Attachment of the LPyV major capsid protein VP1 to receptors on host cells is clearly critical for the restricted tropism of the virus. LPyV VP1 forms a ring-shaped homopentamer in which the five monomers are arranged around a central five-fold axis and connected by extensive interaction surfaces. Sialic acid is a crucial component of the LPyV receptor as removal or modification of cellular sialic acids abolished or modulated LPyV cell binding and infection, but the identity of the sialylated LPyV receptor and its role in tropism are not known. Glycan array and structural analyses show that LPyV VP1 specifically recognizes linear trisaccharides terminating in α2,3-linked sialic acid.

In order to elucidate the carbohydrate-binding specificity of LPyV in a controlled setting, we recombinantly expressed VP1 pentamers that are unable to assemble into capsids due to truncations of 27 and 66 residues at the N- and C-termini, respectively. The LPyV VP1 structure contains one bound Ca2+ ion per chain that is coordinated by the carboxylate group of E46 and the carbonyl group of S214cw as well as several water molecules. In addition, the carboxylate group of E217cw is close enough to the Ca2+ to engage in an ionic interaction. These residues are highly conserved among all polyomaviruses and form one of the two calcium binding sites in the SV40 virion that are important for capsid stability and regulating assembly. While the Ca2+ ions in our structures likely come from the crystallization solution containing 0.2 M calcium chloride, they nevertheless demonstrate that unassembled VP1 pentamers can weakly bind Ca2+ ions. In order to determine whether conformational changes occur in the protein during ligand binding, we compared the complex structures with the unliganded LPyV VP1 structure. In all chains in which the tip of the BC2cw-loop and adjacent residues are not engaged in crystal contacts, the structures are very similar, indicating that the binding site does not undergo a permanent induced fit movement. In two chains, however, a crystal contact perturbed the native structure of the BC2cw-loop, but not the ligand-bound one. Thus, complex formation might stabilize the receptor binding site, and there might be some flexibility in the unbound structure that allows ligand entry into the site. This hypothesis is supported by the B-factors of receptor-binding residues, which are elevated in the unbound structure compared with the complexes.

>[10x]GSHMGGVEVLEVRTGPDAITQIEAYLNPRMGNNIPSEDLYGYSNSINTAFSKASDTPNKDTLPCYSVAVIKLPLLNEDMTCDTILMWEAVSVKTEVVGISSLVNLHQGGKYIYGSSSGCVPVQGTTYHMFAVGGEPLELQGLVASSTATYPDDVVAIKNMKPGNQGLDPKAKALLDKDGKYPVEVWCPDPSKNENTRYYGSFTGGATTPPVMQFTNSVTTVLLDENGVGPLCKGDKLFLSCADIAGVHTNYSETQVWRGLPRYFNVTLRKRIVKNPYP>MIIGYFDGLCEPKNPGGIATFGFVIYLDNRKIEGYGLAEKPFSINSTNNVAEYSGLICLMETMLRLGISSPIIKGDSQLVIKQMNGEYKVKAKRIIPLYEKAIELKKKLNATLIWVPREENKEADRLSRVAYELVRRGKLRDI[2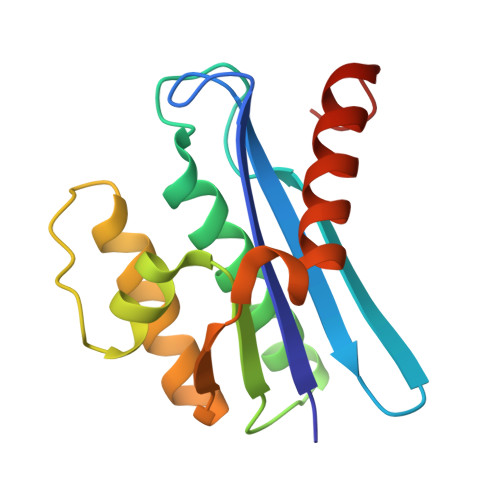x]>MKLVWTLSSWDDYEFWQRTDARMVEKINDLIRNAKRTPFAGLGKPEPLKGDMAGYWSRRITAEHRFVYRVSGSGSEQRLEVIQCRFHYQLEVLFQ[2x]

Type II TA systems are the best understood, and contain both a protein toxin and a more labile protein antitoxin. Many toxins have been identified that degrade RNA, including ribosome-dependent RNase toxins in the RelE family and sub-members YafQ, HigB, and YoeB. Translation inhibition arises from YoeB binding the ribosomal A site and proceeding to cleave mRNA. YoeB toxins conform to a previously characterized RNase fold consisting of two helices packed against a twisted four to five-stranded antiparallel beta sheet.

The structure of the YoeB toxin from A. tumefaciens, herein referred to as AtYoeB, was determined at 1.75 Å resolution. When compared to the EcYoeB toxin, there is an overall RMSD of 0.6 Å for the core residues with 1.2 Å deviation overall. As can be deduced from the protein sequence alignment in Figure 1, these two toxins are 57% identical (76% similar) at the amino acid level, including absolute conservation of the EcYoeB catalytic residues noted in previous studies (blue boxes). The AtYoeB sequence contains four inserted amino acids, located in a loop between beta-strands 4 and 5. This loop was disordered in one of the two copies of AtYoeB present in the crystallographic asymmetric unit; in addition, this loop makes interactions with the tungstate-terillium compound that was critical for bridging important crystal contacts and that was required to obtain usable diffraction quality crystals. The YoeB dimer interface is well conserved among this class of toxin, largely solidified by two tryptophan residues from each monomer (conserved at positions 5 and 10 for both At and EcYoeB) forming an aromatic ring cluster, in addition to polar interactions mediated by conserved Tyr13, Gln17 and Asn18 side chains. Additional interactions are noted for AtYoeB at positions that differ from its Ec counterpart: (Ec to At) Leu14Glu, Glu18Arg, and Lys32Arg. These changes generate additional polar interactions for the AtYoeB dimer. Examination of sequence variants and available structures pointed to a four amino acid helix that varies in sequence and appears to make important contacts with the first base of the mRNA codon in the ribosome.> GLFDAPGRSQFVPADQAFAFDFQQNQHDLNLTWQIKDGYYLYRKQIRITPEHAKIADVQLPQGVWHED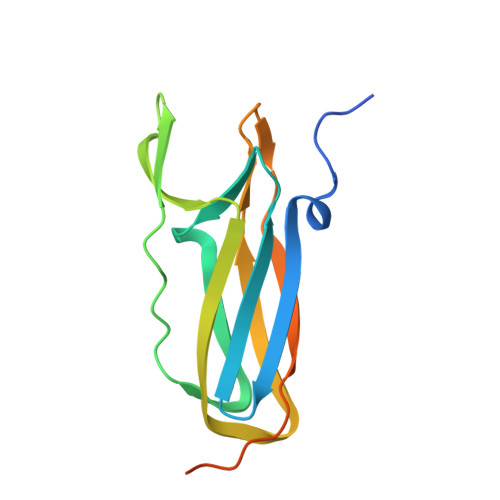EFYGKSEIYRDRLTLPVTINQASAGATLTVTYQGSADAGFCYPPETKTVPLSEVVANNAAPQPVSVPQQEQPTAQ N-[(S)-({[(benzyloxy)carbonyl]amino}methyl)(hydroxy)phosphoryl]-L-leucyl-L-valine 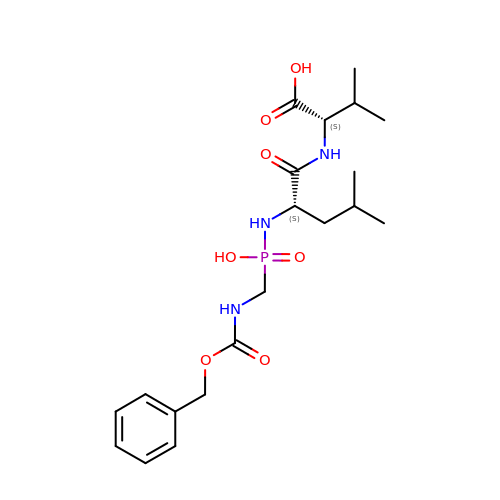| C20 H32 N3 O7 P | VYQPALSHFDHUJW-IRXDYDNUSA-N> MPSNQEARLFLAVLVLAQVLPILVDSAAEKGFKQAFWQPLCQVSEELDDQPKGALFTLQAAASKIQKMRDAALRASIYAEINHGTNRAKAAVIVANHYAMKADSGLEALKQTLSSQEVTATATASYLKGRIDEYLNLLLQTKESGTSGCMMDTSGTNTVTKAGGTIGGVPCKLQLSPIQPKRPAATYLGKAGYVGLTRQADAANNFHAAAAECRLASGHNTNGLGKSGQLSAAV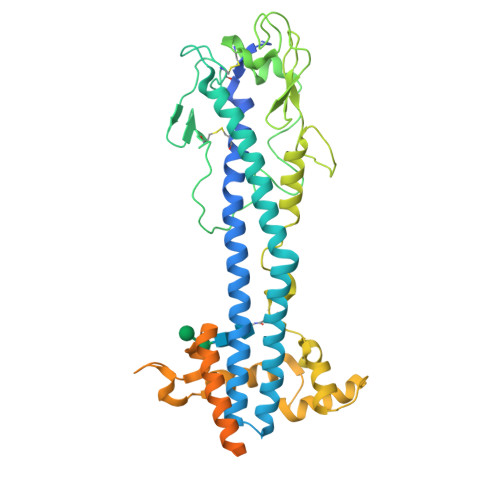TMAAGYVTVANSQTAVTVQALDALQEASGAAHQPWIDAWKAKKALTGAETAEFRNETAGIAGKTGVTKLVEEALLKKKDSEASEIQTELKKYFSGHENEQWTAIEKLISEQPVAQNLVGDNQPTKLGELEGNAKLTTILAYYRMETAGKFEVLTQKHKPAESQQQAAETEGSCNKKDQNECKSPCKWHNDAENKKCTLDKEEAKKVADETAKDGKTGNTNTTGSSNSFVISKTPLWLAVLLF> MELALALSLIASVAAAPTATLANGDTITGLNAIINEAFLGIPFAEPPVGNLRFKDPVPYSGSLDGQKFTSYGPSCMQQNPEGTYEENLPKAALDLVMQSKVFEAVSPSSEDCLTINVVRPPGTKAGANLPVMLWIFGGGFEVGGTSTFPPAQMITKSIAMGKPIIHVSVNYRVSSWGFLAGDEIKAEGSANAGLKDQRLGMQWVADNIAAFGGDPTKVTIFGESAGSMSVMCHILWNDGDNTYKGKPLFRAGIMQSGAMVPSDAVDGIYGNEIFDLLASNAGCGSASDKLACLRGVSSDTLEDATNNTPGFLAYSSLRLSYLPRPDGVNITDDMYALVREGKYANIPVIIGDQNDEGTFFGTSSLNVTTDAQAREYFKQSFVHASDAEIDTLMTAYPGDITQGSPFDTGILNALTPQFKRISAVLGDLGFTLAR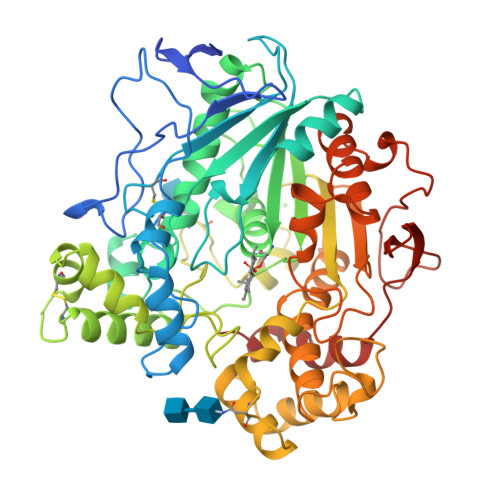RYFLNHYTGGTKYSFLSKQLSGLPVLGTFHSNDIVFQDYLLGSGSLIYNNAFIAFATDLDPNTAGLLVKWPEYTSSSQSGNNLMMINALGLYTGKDNFRTAGYDALFSNPPSFFV>[4x]GPHMEHNYEDIAQEFIDFIYKNPTTYHVVSFFAELLDKHNFKYLSEKSNWQDSIGEDGGKFYTIRNGTNLSAFILGKNWRAEKGVGVIGSHVDALTVKLKPVSFKDTAEGYGRIAVAPYGGTLNELW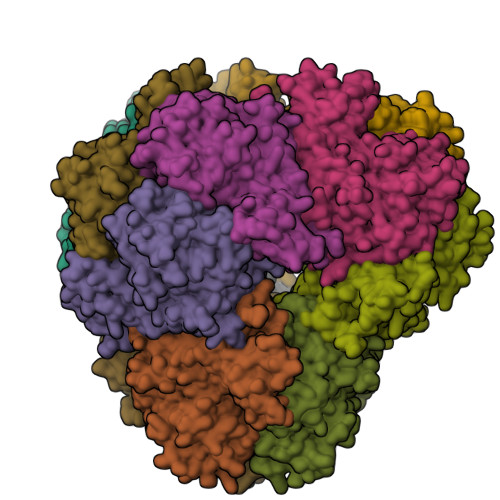LDRDLGIGGRLLYKKKGTNEIKSALVDSTPLPVCRIPSLAPHFGKPAEGPFDKEDQTIPVIGFPTPDEEGNEPPTDDEKKSPLFGKHCIHLLRYVAKLAGVEVSELIQMDLDLFDVQKGTIGGIGKHFLFAPRLDDRLCSFAAMIALICYAKDVNTEESDLFSTVTLYDNEEIGSLTRQGAKGGLLESVVERSSSAFTKKPVDLHTVWANSIILSADVNHLYNPNFPEVYLKNHFPVPNVGITLSLDPNGHMATDVVGTALVEELARRNGDKVQYFQIKNNSRSGGTIGPSLASQTGARTIDLGIAQLSMHSIRAATGSKDVGLGVKFFNGFFKHWRSVYDEFGEL>[2x]GPDSMSEGFSSSSIQELYQSLKEITNNADVELFEDRITKLDFESTDEPKHANDIIKDRFLRPSNALPWSLLDMVQDVPHTSSPEDCSGKLDYKELLKVPDPINRTSYQFKRTGLEGKISGYKEEVDLKEVANANASNSLSITRSINHNQNSVRGSTAQLPFTPGGIPMKSVKTDSEQNGSSTMANATKLLHKDGQGLFDIPEGMNRGIKPMDXXXXXXXXXXXXXXXXXXXXXXXXXXXXXXXXXXXXXXXXXXXXXXXXXXXXXXXXXXXXXXXXXXXXXXXXXXXXXXXXXXXXXXXXXXXXEWAHVVDLNHKIENFDELIPNPARSWPFELDTFQKEAVYHLEQGDSVFVAAHTSAGKTVVAEYAIAMAHRNMTKTIYTSPIKALSNQKFRDFKETFDDVNIGLITGDVQINPDANCLIMTTEILRSMLYRGADLIRDVEFVIFDEVHYVNDQDRGVVWEEVIIMLPQHVKFILLSATVPNTYEFANWIGRTKQKNIYVISTPKRPVPLEINIWAKKELIPVINQNSEFLEANFRKHKEILNGESAKGAPSKTDNGRGGSTARGGRGGSNTRDGRGGRGNSTRGGANRGGSRGAGAIGSNKRKFFTQDGPSKKTWPEIVNYLRKRELLPMVVFVFSKKRCEEYADWLEGINFCNNKEKSQIHMFIEKSITRLKKEDRDLPQILKTRSLLERGIAVHHGGLLPIVKELIEILFSKGFIKVLFATETFAMGLNLPTRTVIFSSIRKHDGNGLRELTPGEFTQMAGRAGRRGLDSTGTVIVMAYNSPLSIATFKEVTMGVPTRLQSQFRLTYNMILNLLRIEALRVEEMIKYSFSENAGSRGLSLLPDYEKRLAVLKDTEFIDQNHNVLLKGRVACEINSGYELVLTELILDNFLGSFEPEEIVALLSVFVYEGKTREEEPPIVTPRLAKGKQRIEEIYKKMLCVFNTHQIPLTQDEAEFLDRKRFAMMNVVYEWARGLSFKEIMEMSPEAEGTVVRVITWLDEICREVKTASIIIGNSTLHMKMSRAQELIKRDIVFAASLYL;>[2x]GPDSMSDIKQLLKEAKQELTNRDYEETIEISEKVLKLDPDNYFAHIFLGKALSSLPASNNVSSNRNLERATNHYVSAAKLVPDNLLAWKGLFLLFRTTEVVPDILSYDEYFDLCGQYADALLKQEQSQVELINDIKLLKKTHPDCQKAFYQHLKPGSLMAETIGRHLSTP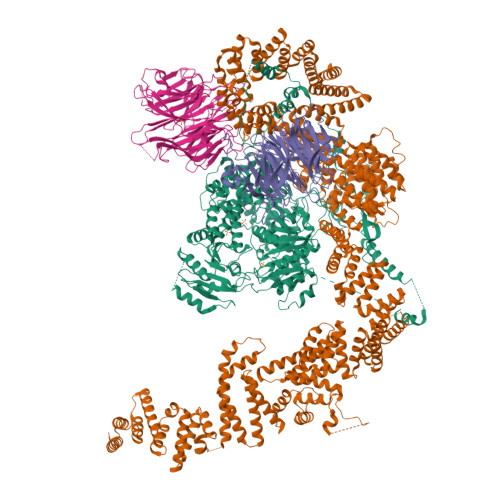QDALLNLIKILSNIETTEIGKTLSQNRLKLKASDPDYQIKLNSFSWEIIKNSEIDQLYNQLVNILADDQKRSEIENQWLEYRIKVLKSMPLDVKKDFFTKVKEMVEDMVLVNHQSLLAWQKYFEWTDYEDLDNMDAPLIIKYFKKFPKDPLAMILYSWLSSKLSKYDIKSLESANKPPEGHKKTEKETDIKDVDETNEDEVKDRVEDEVKDRVEDEVKDQDEEAKEDEEEDLDDIEIGLLEEEVVTVLTENIVKCKNNILAHRILCQYYLLTKEYEAALPYIKNGISLIAYNIKDLGVHLPLTKREFSLDLATVYTYVDAPKDHNAALKLYDNILSGDFSNIQAKMGKGIIFIERKNWKDAMTLLTQVHEQSPNNLEVLSELSWSKAHMGYMDEALAGLDTVIKGIKGMDLRSIDFRALNLWRQAKVYIMKHASINDAKQENVKCAFKLLIQSIKILDTFAPGFSTLGDIYCHYYKDHLRAFKCYFKAFDLDAGDYTAAKYITETYASKPNWQAASSIASRLIKGEKAKAELRSNNWPFRVVGIAHLEKQEESDSIEWFQSALRVDPNDVESWVGLGQAYHACGRIEASIKVFDKAIQLRPSHTFAQYFKAISLCDVGEYLESLDILEKVCQEAATEESFQIGLVEVLMRCSLDLYSQGFLLKSVSIAKDTIERIKIIISELKCENQQVWIYLSQVLRLFIWIESKVDTLPVESLVSIFENSQFSGSEEIDSVDNIKIDTLLDSTTDDNVSIACKFLILASKYSVSDQKFTDIAGTVRASYWYNIGISELTAFITLKEPQYRDAAIFAFKKSIQLQSNTSETWIGLGIATMDINFRVSQHCFIKATALEPKATNTWFNLAMLGLKKKDTEFAQQVLNKLQSLAPQDSSPWLGMALILEEQGDIIGSSKLFAHSFILSNGRSKAAQFMYAKNVLENHINNGDDERDIETVEKLTTASIALEQFFKKSPDSQFALQCALLTLERLHHYENANELANRLIGILEKKFEKTQDERELFNFAIIKGQFARIHLGLGNFELSIENADLSQGIISESSDEKSMKTKISNHICLGLSYFFLNDFDQTLNQFQELLSISKDSKHLVVLIAKVLYDVGESDTKEIALQELTEYIATSGADLLVTLTIAAMSILDDKREDLSIILEELKALPLSKQIIDKHKDAPYLIEEITKRLYRNDTGKQVWQRSAYFFPNNLKVWERLDKNIQRRIASNGQNKVTAEEMSKLYCESKNLRSIQRGMFLCPWNVTAVKALNECF;>[4x]MSKVFIATANAGKAHDADIFSVSACNSFTVSCSGDGYLKVWDNKLLDNENPKDKSYSHFVHKSGLHHVDVLQAIERDAFELCLVATTSFSGDLLFYRITREDETKKVIFEKLDLLDSDMKKHSFWALKWGASNDRLLSHRLVATDVKGTTYIWKFHPFADESNSLTLNWSPTLELQGTVESPMTPSQFATSVDISERGLIATGFNNGTVQISELSTLRPLYNFESQHSMINNSNSIRSVKFSPQGSLLAIAHDSNSFGCITLYETEFGERIGSLSVPTHSSQASLGEFAHSSWVMSLSFNDSGETLCSAGWDGKLRFWDVKTKERITTLNMHCDDIEIEEDILAVDEHGDSLAEPGVFDVKFLKKGWRSGMGADLNESLCCVCLDRSIRWFREAGGK>[2x]ALYEDPPDQKTSPSGKPATLKIASWNVDGLRAWIKKKGLDWVKEEAPDILCLQETKCSENKLPAELQELPGLSHQYWSAPSDKEGYSGVGLLSRQCPLKVSYGIGDEEHDQEGRVIVAEFDSFVLVTAYVPNAGRGLVRL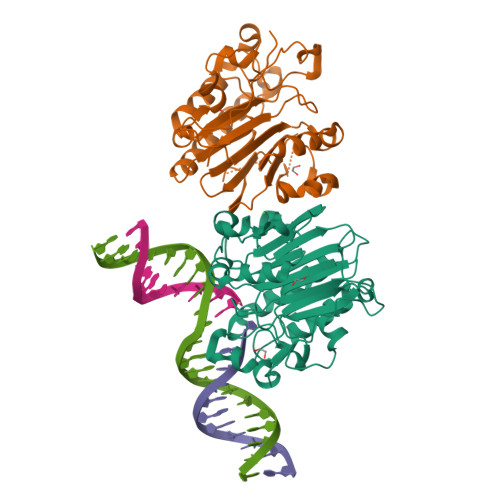EYRQRWDEAFRKFLKGLASRKPLVLCGDLNVAHEEIDLRNPKGNKKNAGFTPQERQGFGELLQAVPLADSFRHLYPNTPYAYTFWTYMMNARSKNVGWRLDYFLLSHSLLPALCDSKIRSKALGSDHCPITLYLAL>GSHMASLQKTRIINSMLQAAAGKPVNFKEMAE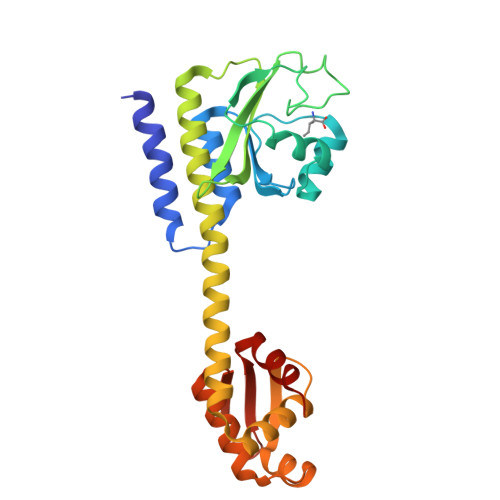TLRDVIDSNIFVVSRRGKLLGYSINQQIENDRMKKMLEDRQFPEEYTKNLFNVPETSSNLDINSEYTAFPVENRDLFQAGLTTIVPIIGGGERLGTLILSRLQDQFNDDDLILAEYGATVVGMEILREKAEEIEEEARSKAVVQMAISSLSYSELEAIEHIFEELDGNEGLLVASKIADRVGITRSVIVNALRKLESAGVIESRSLGMKGTYIKVLNNKFLIELENLKSH[4x]>[3x]CSEVISVTSTEEVCTIQENKETCTFNHATTITLQPLQQQTCLTLNDPEKRPMGMLTVKPDGIKFRCNKKIEFFTRDHQIVSESVHRCHRAGSCHSDECHHVKDTDALPEFSSEANSRPGYTSCSSSCGC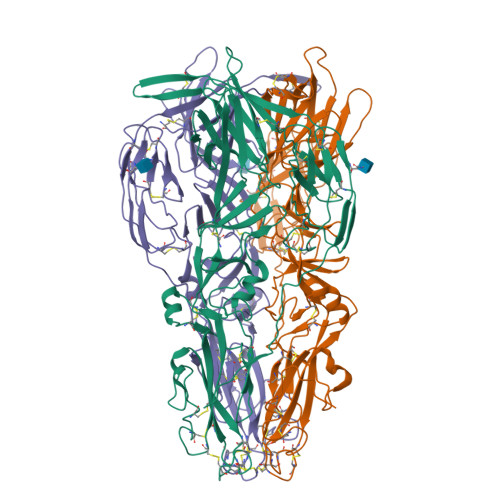ITCDGCFFCEPSCLFHRLYAIPTTPTIYSIFYCPSWELEVDAEISLQREDETTTSTIRLLPGRTSTWNNIRFSLIGTIVPQLPILSSAFVTNGRQTSIVKPAYAGQLQSNSVGQLQCPNLEAAKQFECHFSRNLCTCTNALHKVSCTCYDGSVEDHMEALPLPQTSKNFLVFEKDRNIYAKTHVGSALQLHIVAQDLKITTVKHTSHCQVEASDLSGCYSCTSGASLTLSCKSDNGEVLANMKCNEQTHVIRCTESGFINNILLMFDTSEVAADCTAACPGGIVNFTIKGLLAFVNERIISQSYSATDVERNIKGKPIPNPLLGLDSTRTGHHHHHH> 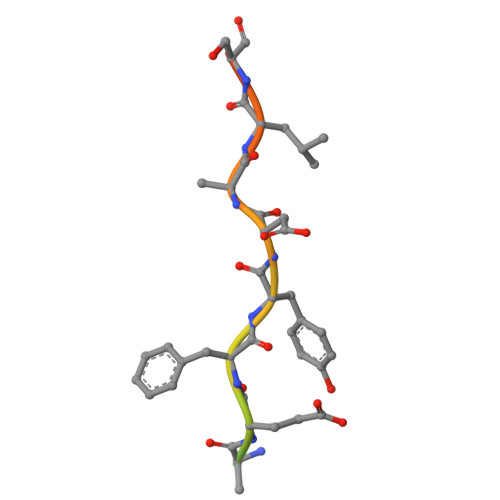GAMRSILSEDEFYDALSDSES>ASRYLTDMTLEEMSRDWFMLMPKQKVAGSLCIRMDQAIMDKNIILKANFSVIFDRLETLILLRAFTEEGAIVGEISPLPSLPGHTDEDVKNAVGVLIGGLEANDNTVRVSET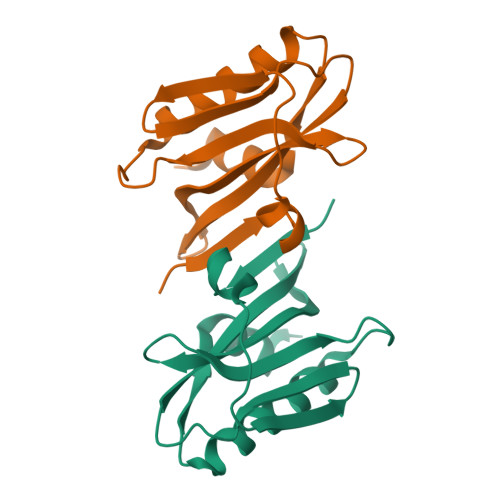LQRFAWRS[2x]> GSSRAMGNEVAGVEDISVEIKPSSKRNSDARRTSRNVCSNEERKRRKYFHMLYLVCLMVHGFIRNEWINSKRLSRKLSNLVPEKVFELLHPQKDEELPLRSTRKLLDGLKKCMELWQKHWKITKKYDNEGLYMRTWKEIEMSANNKRKFKTLKRSDFLRAVSKGHGDPDISVQGFVAMLRACNVNARLIMSCQPPDFTNMKIDTSLNGNNAYKDMVKYPIFWCEVWDKFSKKWITVDPVNLKTIEQVRLHSKLAPKGVACCERNMLRYVIAYDRKYGCRDVTRRYAQWMNSKVRKRRITKDDFGEKWFRKVITALHHRKRTKIDDYEDQYFFQRDESEGIPDSVQDLKNHPYYVLEQDIKQTQIVKPGCKECGYLKVHGKVGKVLKVYAKRDIADLKSARQWYMNGRILKTGSRCKKVIKRTVGRPKGEAEEEDERLYSFEDTELYIPPLASASGEITKNTFGNIEVFAPTMIPGNCCLVENPVAIKAARFLGVEFAPAVTSFK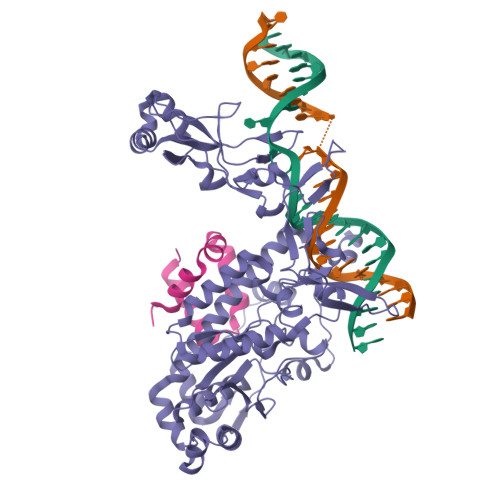FERGSTVKPVLSGIVVAKWLREAIETAIDGIEFI;> GSGNASSGALGTTGGATDAAQGGPPGSIGLTVEDLLSLRQVVSGNPEALAPLLENISARYPQLREHIMANPEVFVSMLLEAVGDNMQDVMEGADDMVEGEDIEVTGEAAAAGLGQGEGEGSFQVDYTPEDDQAISRLCELGFERDLVIQVYFACDKNEEAAANILFSDHAD>[2x]SLKNEELYHQSYDCVCVMFASIPDFKEFY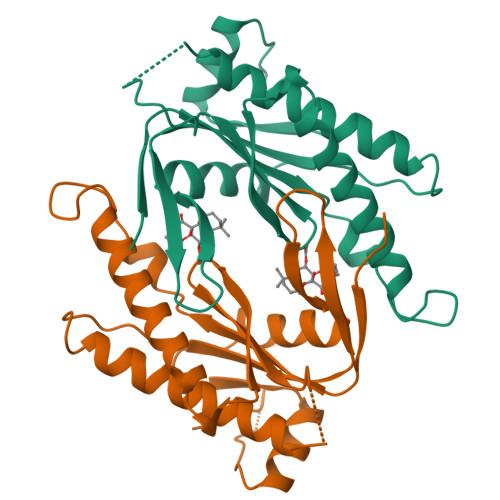TESDVNKEGLECLRLLNEIIADFDDLLSKPKFSGVEKIKTIGSTYMAATGLSAIPSQEHAQEPERQYMHIGTMVEFAYALVGKLDAINKHSFNDFKLRVGINHGPVIAGVIGAQKPQYDIWGNTVNVASRMDSTGVLDKIQVTEETSLILQTLGYTCTCRGIINVKGKGDLKTYFVNTEMSRSLSQSNLAS> GVSGSCNIDVVCPEGDGRRDIIRAVGAYSKSGTLACTGSLVNNTANDRKMYFLTAHHCGM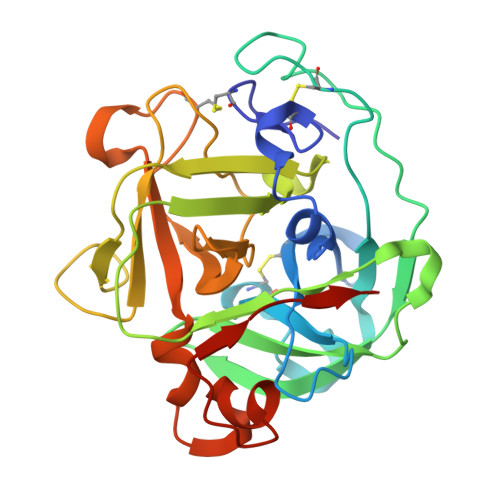GTASTAASIVVYWNYQNSTCRAPNTPASGANGDGSMSQTQSGSTVKATYATSDFTLLELNNAANPAFNLFWAGWDRRDQNYPGAIAIHHPNVAEKRISNSTSPTSFVAWGGGAGTTHLNVQWQPSGGVTEPGSSGSPIYSPEKRVLGQLHGGPSSCSATGTNRSDQYGRVFTSWTGGGAAASRLSDWLDPASTGAQFIDGLDSGGGTP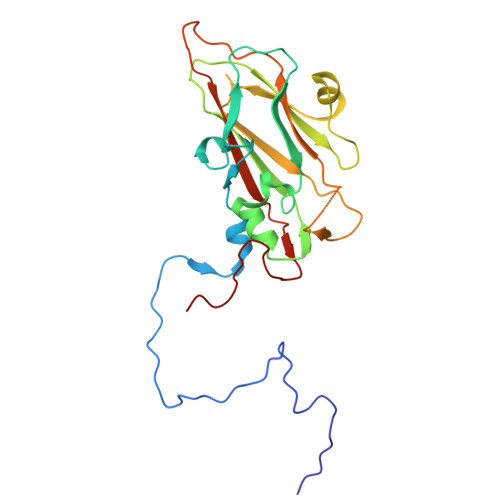> GLPTMLTPGSNQFLTSDDFQSPSAMPQFDVTPEMDIPGQVNNLMEIAEVDSVVPVNNTEGKVLSIESYQIPVQSNSTNGSQVFGFPLMPGASSVLNRTLLGEILNYYTHWSGSIKLTFMFCGSAMATGKFLLAYSPPGAGAPTTRKEAMLGTHVIWDVGLQSSCVLCIPWISQTHYRYVVVDEYTAGGYITCWYQTNIVVPADTQSDCKILCFVSACNDFSVRMLKDTPFIKQDNFYQ>AGFQLNEFSSSGLGRAYSGEGAIADDAGNVSRNPALITMFDRPTFSAGAVYIDPDVNISGTSPSGRSLKADNIAPTEWVPNMHFVAPINDQFGWGASITRNYGLATEFNDTYAGGSVGGTTDLETMNLNLSGAYRLNNAWSFGLGFNAVYARAKIERFAGDLGQLVAGQIMQSPAGQTQQGQALAATANGIDSNTKIAHLNGNQWGFGWNAGILYELDKNNRYALTYRSEVKIDFKGNYSSDLNRAFNNYGLPIPTATGGATQSGYLTLNLPEMWEVSGYNRVDPQWAIHYSLAYTSWSQFQQLKATSTSGDTLFQKHEGFKDAYRIALGTTYYYDDNWTFR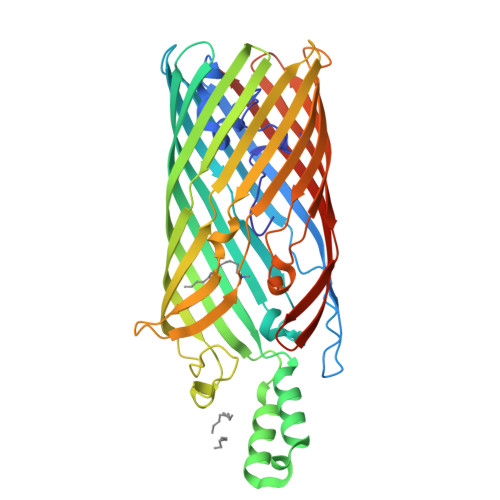TGIAFDDSPVPAQNRSISIPDQDRFWLSAGTTYAFNKDASVDVGVSYMHGQSVKINEGPYQFESEGKAWLFGTNFNYAFHHHHHH[2x]> SKELRQLQEDRKNDKKPPPYKHIKVNRPIGRVQIFTADLSEIPRCNCKATDENPCGIDSECINRMLLYECHPTVCPAGGRCQNQCFSKRQYPEVEIFRTLQRGWGLRTKTDIKKGEFVNEYVGELIDEEECRARIRYAQEHDITNFYMLTLDKDRIIDAGPKGNYARFMNHCCQPNCETQKWSVNGDTRVGLFALSDIKAGTELTFNYNLECLGNGKTVCKCGAPN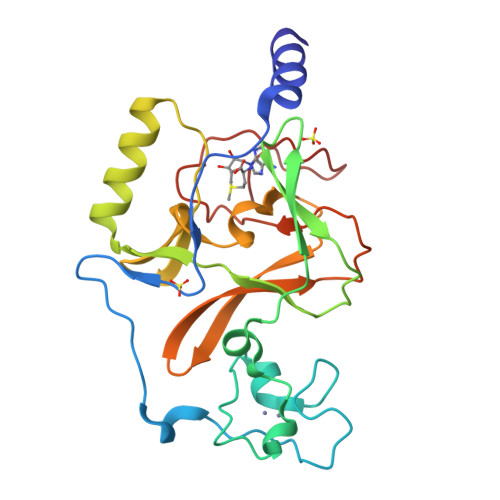CSGFLG> GMVLEATMICIDNSEWMRNGDYSPSRLQAQTEAVNLLCGAKTQSNPENTVGILTMAGKGVRVLTTPTSDLGKILACMHGLDVGGEINLTAAIQIAQLALKHRQNKNQRQRIIVFAGSPIKYEKKALEIVGKRLKKNSVSLDIVNFGEDDDEEKP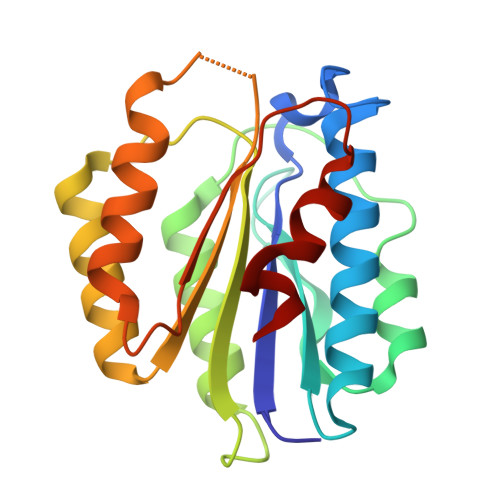QKLEALLTAVNNNDGSHIVHVPSGANALSDVLLSTPVFTG>[6x]GSTAPPTNQWYHGKLDRTIAEERLRQAGKSGSYLIRESDRRPGSFVLSFLSQMNVVNHFRIIAMSGDYYIGGRRFSSLSDLIGYYSHVSSLLKGEKLLYPVAPPEPVED

p120RasGAP is a multidomain regulator of Ras signaling, containing two SH2 domains at its N-terminus and multiple other domains including a RasGAP. Binding of p190RhoGAP is mediated by phosphotyrosine-SH2 domain interactions, and a major driver is thought to be between the N-terminal SH2 of p120RasGAP and pTyr-1105 of p190RhoGAP. p190RhoGAP recruitment has multiple effects, including inhibition of Rho signaling by locating p190RhoGAP to the plasma membrane, and activation of Ras signaling by suppression of p120RasGAP’s RasGAP activity when it is bound to p190RhoGAP. Therefore, in this study we determine the crystal structures of the N-terminal SH2 domain of p120RasGAP alone, and its complex with a phosphorylated peptide corresponding to residues around and including pTyr-1105 of p190RhoGAP. The SH2 fold consists of a central β-sheet flanked by two α-helices, and both crystal structures reveal that the p120RasGAP N-terminal SH2 domain adopts this fold.

We began by expressing and purifying the N-terminal SH2 domain of p120RasGAP alone, and by obtaining apo crystals of this domain. These crystals diffracted well, and we obtained a 1.75 Å dataset that contains 6 copies per asymmetric unit. Of the 6 copies, chains A and B show significantly lower B-factors and improved electron density compared to the other copies and we have based our analyses on these chains. In our crystal structure of apo p120RasGAP, we observe six copies per asymmetric unit arranged as dimers (chains A/B, C/D, E/F). Superposition of the crystallographic dimers reveals that there are two conformational classes, which can be defined by the conformation of the βG and βE-βF loops. Interestingly, these loops important for specificity determination at the +3 position of the phosphopeptide. We observe that in one class the loops are open and poised for peptide binding, and in the other they are closer and seem to occlude peptide binding. In both classes, the B-factors of βG loop are high, and in the occluded form this loop cannot be built in two of the three copies, however, when the bound phosphopeptide structure is superposed on these conformations the occluded state clashes with His-1109 at peptide position +4, but the poised conformation can accommodate binding. We interpret this to indicate conformational flexibility and sampling of the specificity defining loops in the absence of phosphopeptide binding. In the apo structure, we do not observe a similar orientation of arginines, Arg-231 and Arg-212, we therefore infer the cation-π stack to be induced by peptide binding.>FHKIRNEDLIFNESLGQGTFTKIFKGVRREVGDYGQLHETEVLLKVLDKAHRNYSESFFEAASMMSKLSHKHLVLNYGVCFCGDENILVQEFVKFGSLDTYLKKNKNCINILWKLEVAKQLAAAMHFLEENTLIHGNVCA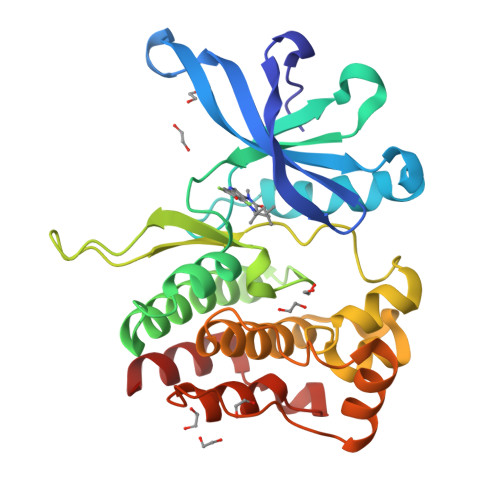KNILLIREEDRKTGNPPFIKLSDPGISITVLPKDILQERIPWVPPECIENPKNLNLATDKWSFGTTLWEICSGGDKPLSALDSQRKLQFYEDRHQLPAPKAAELANLINNCMDYEPDHRPSFRAIIRDLNSL[2x]>DGGFC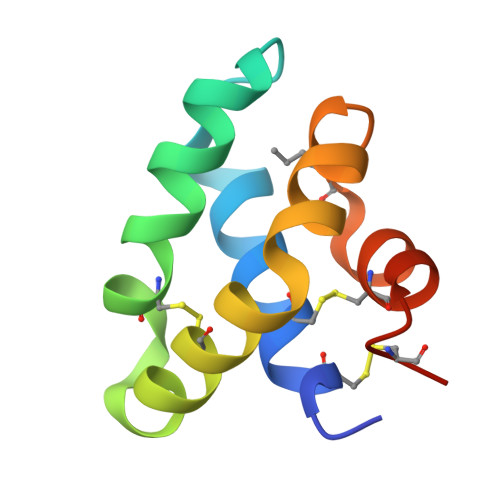EVCKKLVGYLDRNLEKNSTKQEILAALEKGCSFLPDPYQKQCDQFVAEYEPVLIEILVEVLDPSFVCLKIGACPSAH[2x]>GAQKKTQKTYIPWSNGKLVVSEEGRYLKHENGTPFFWLGETGWLLPERLNRDEAEYYLEQCKRRGYNVIQVQTLNNVPSMNIYGQYSMTDGYNFKNINQKGVYGYWDHMDYIIRTAAKKGLYIGMVCIWGSPVSHGEMNVDQAKAYGKFLAERYKDEPNIIWFIGGDIRGDVKTAEWEALATSIKAIDKNHLMTFHPRGRTTSATWFNNAPWLDFNMFQSGHRRYGQRFGDGDYPIEENTEEDNWRFVERSMAMKPMKPVIDGEPIYEEIPHGLHDENELLWKDYDVRRYAYWSVFAGSFGHTYGHNSIMQFIKPGVGGAYGAKKPWYDALNDPGYNQMKYLKNLMLTFPFFERVPDQSVIAGQNGERYDRAIATRGNDYLMVYNYTGRP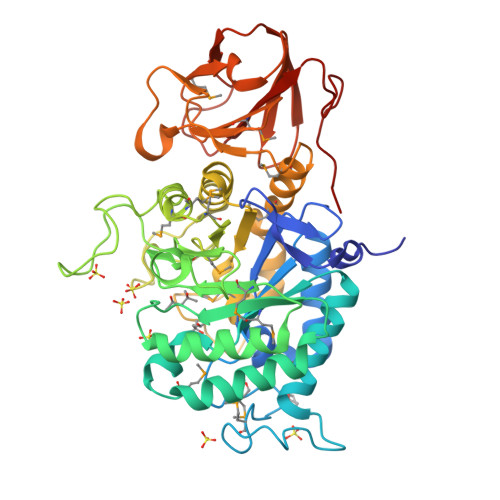MEVDFSKISGAKKNAWWYTTKDGKLEYIGEFDNGVHKFQHDSGYSSGNDHVLIVVDSSKDYVKKDCYQIDTHE[4x]Here, a novel and rapid method to obtain experimental phases for protein structure determination by vanadium phasing is reported. Vanadate is a transition-state mimic of phosphoryl-transfer reactions and it has the advantage of binding specifically to the active site of numerous enzymes catalyzing this reaction. The applicability of vanadium phasing has been validated by determining the structures of three different protein–vanadium complexes, two of which are integral membrane proteins: the rabbit sarcoplasmic reticulum Ca2+-ATPase, the antibacterial peptide ATP-binding cassette transporter McjD from Escherichia coli and the soluble enzyme RNAse A from Bos taurus. In order to test whether vanadium can indeed be used for experimental phasing, we collected long-wavelength X-ray diffraction data from three known protein–vanadate complexes for V-SAD phasing: two membrane-transport proteins, the antibacterial peptide ATP-binding cassette (ABC) transporter McjD from E. coli and the rabbit sarcoplasmic reticulum Ca2+-ATPase (SERCA; Clausen et al., 2016), and a soluble enzyme, bovine pancreatic ribonuclease A (RNAseA; Ladner et al., 1997).

SERCA is a larger membrane protein of 110 kDa that belongs to the family of P-type ATPases. Its function during muscle relaxation is to pump Ca2+ from the cytosol to the sarcoplasmic reticulum at the expense of ATP hydrolysis. In contrast to the tetrahedral VO4 form bound to McjD, the vanadate species bound to SERCA has been modeled in its trigonal planar VO3 state, mimicking the pentacovalent transition state of dephosphorylation. SERCA–VO3 crystallizes in space group P21, with two monomers per asymmetric unit, each of which binds one VO3 ion. The crystals diffracted to 3.1 Å resolution, and despite a ratio of one vanadium per 994 protein residues, both of the V atoms could be located. The automatic structure-determination pipeline CRANK2 was also able to locate some of the S atoms in addition to the vanadium sites and built an initial model (1690 out of 1988 residues). The sulfur positions were essential to obtain interpretable electron-density maps [Fig. 1(b) and Supplementary Fig. S2], which explains why a higher redundancy of 77 was needed to improve the initial phases. Iterative cycles of manual model building and refinement, further aided by the sulfur peaks in the anomalous difference Fourier maps using the phases from the evolving model, allowed a full structure determination. The final structure had an overall all-atom r.m.s.d. of 0.6 Å compared with the previously reported SERCA–VO3 structure determined by molecular replacement. Analysis of the SERCA data sets showed that at least four data sets were necessary to obtain an initial model using the automatic phasing pipeline.

>MEAAHSKSTEECLAYFGVSETTGLTPDQVKRHLEKYGHNELPAEEGKSLWELVIEQFEDLLVRILLLAACISFVLAWFEEGEETITAFVEPFVILLILIANAIVGVWQERNAENAIEALKEYEPEMGKVYRADRKSVQRIKARDIVPGDIVEVAVGDKVPADIRILSIKSTTLRVDQSILTGESVSVIKHTEPVPDPRAVNQDKKNMLFSGTNIAAGKALGIVATTGVSTEIGKIRDQMAATEQDKTPLQQKLDEFGEQLSKVISLICVAVWLINIGHFNDPVHGGSWIRGAIYYFKIAVALAVAAIPEGLPAVITTCLALGTRRMAKKNAIVRSLPSVETLGCTSVICSDKTGTLTTNQMSVCKMFIIDKVDGDFCSLNEFSITGSTYAPEGEVLKNDKPIRSGQFDGLVELATICALCNDSSLDFNETKGVYEKVGEATETALTTLVEKMNVFNTEVRNLSKVERANACNSVIRQLMKKEFTLEFSRDRKSMSVYCSPAKSSRAAVGNKMFVKGAPEGVIDRCNYVRVGTTRVPMTGPVKEKILSVIKEWGTGRDTLRCLALATRDTPPKREEMVLDDSSRFMEYETDLTFVGVVGMLDPPRKEVMGSIQLCRDAGIRVIMITGDNKGTAIAICRRIGIFGENEEVADRAYTGREFDDLPLAEQREACRRACCFARVEPSHKSKIVEYLQSYDEITAMTGDGVNDAPALKKAEIGIAMGSGTAVAKTASEMVLADDNFSTIVAAVEEGRAIYNNMKQFIRYLISSNVGEVVCIFLTAALGLPEALIPVQLLWVNLVTDGLPATALGFNPPDLDIMDRPPRSPKEPLISGWLFFRYMAIGGYVGAATVGAAAWWFMYAEDGPGVTYHQLTHFMQCTEDHPHFEGLDCEIFEAPEPMTMALSVLVTIEMCNALNSLSENQSLMRMPPWVNIWLLGSICLSMSLHFLILYVDPLPMIFKLKALDLTQWLMVLKISLPVIGLDEILKFIARNYLEG[2x]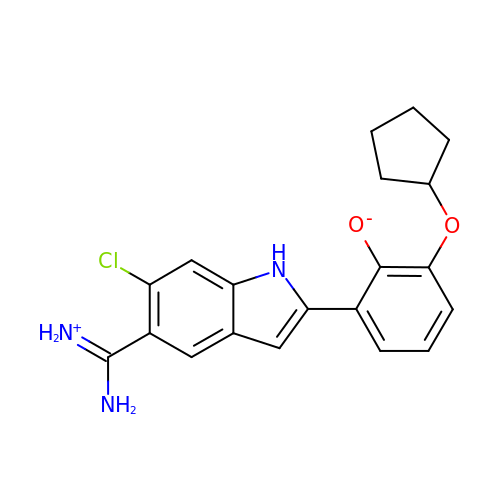2-{5-[AMINO(IMINIO)METHYL]-6-CHLORO-1H-INDOL-2-YL}-6-(CYCLOPENTYLOXY)BENZENOLATE | C20 H20 Cl N3 O2 | QXAURVOBXQBPAP-UHFFFAOYSA-N>[4x]MRGSHHHHHHTDPMSVIKPDMKIKLRMEGAVNGHPFAIEGVGLGKPFEGKQSMDLKVKE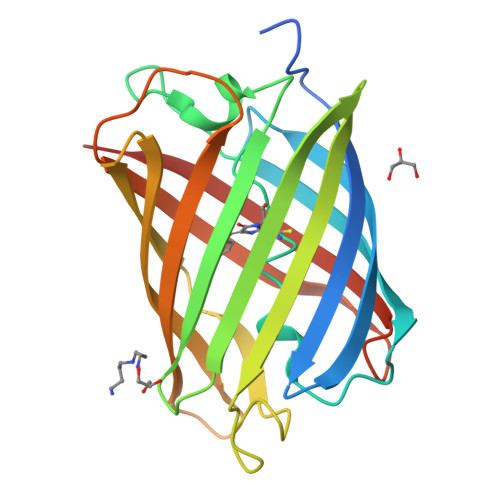GGPLPFAYDILTMAFCYGNRVFAKYPENIVDYFKQSFPEGYSWERSMIYEDGGICNATNDITLDGDCYICEIRFDGVNFPANGPVMQKRTVKWELSTEKLYVRDGVLKSDGNYALSLEGGGHYRCDFKTTYKAKKVVQLPDYHSVDHHIEIISHDKDYSNVNLHEHAEAHSELPRQAK>GMSAGKTVVIALGGNAMLQAKEKGDYDTQRKNVEIAASEIYKIHKAGYKVVLTSGNGPQVGAIKLQNQAAAGVSPEMPLHVCGAMSQGFIGYMMSQAMDNVFCANNEPANCVTCVTQTLVDPKDQAFTNPTKPVGRFYTEQEAKDLMAANPGKILREDAGRGWRVVVPSPRPLEIVEYGVIKTLIDNNVLVICTNGGGIPCKRENKVISGVDAVIDKDLATSLLAKTLNSDYLMILTDVLNACINYKKPDERKLEEIKLSEILALEKDGHFAAGSMGPKV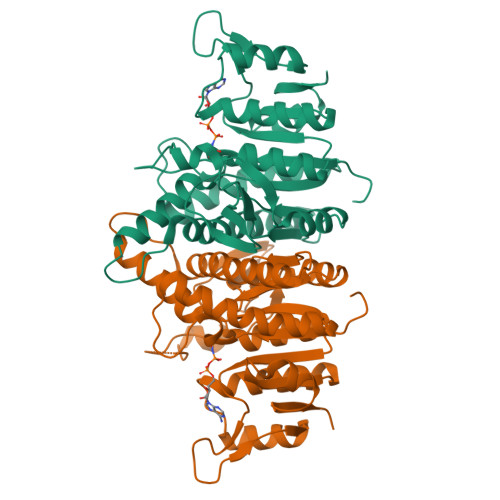RAAIEFTQATGKMSIITSLSTAVDALNGKCGTRIIKD[4x]>[6x]MSLIRIGHGFDVHAFGEDRPLIIGGVEVPYHTGFIAHSDGDVALHALTDAILGAAALGDIGKLFPDTDMQ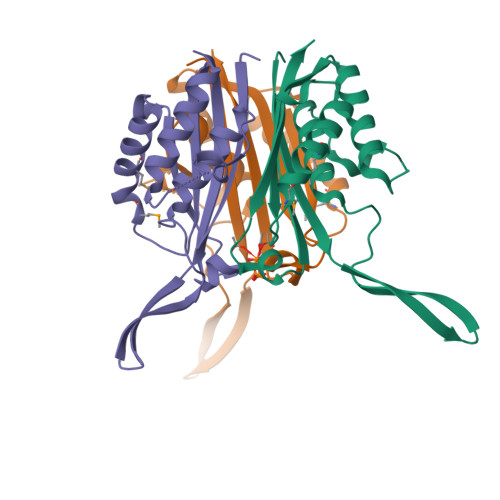YKNADSRGLLREAFRQVQEKGYKIGNVDITIIAQAPKMRPHIDAMRAKIAEDLQCDIEQVNVKATTTEKLGFTGRQEGIACEAVALLIRQEGGSHHHHHH Glutathione transferases (GSTs) constitute a widespread superfamily of enzymes notably involved in detoxification processes and/or in specialized metabolism. In the cyanobacterium Synechocsytis sp. PCC 6803, SynGSTC1, a chi-class GST (GSTC), is thought to participate in the detoxification process of methylglyoxal, a toxic by-product of cellular metabolism. GSTCs were shorter of about 30 residues compared to most cytosolic GSTs and had a well-conserved SRAS motif in the active site (10SRAS13 in SynGSTC1). The crystal structure of SynGSTC1 in complex with glutathione adopted the canonical GST fold with a very open active site because the α4 and α5 helices were exceptionally short.

We also solved the structures of two variants (S10T and R11A variants in complex with GSH) which did not show significant differences from the wild-type. The R11A substitution also did not fully abolish the activity of the enzyme even though it decreased significantly (divided by a factor close to 250 as compared to WT). R11 formed a salt bridge with the N-terminal carboxylate group of GSH in the crystal structure (see above in Section 3.3). The electrostatic influence of R11 on the catalytic process was, however, clear since the catalytic rate was 75 times lower in R11A compared to WT. This was accompanied by a significant one-unit increase in optimal pH suggesting a higher GSH-thiol pKa in the R11A variant than in the WT enzyme. The SynGSTC1 residues with the largest contributions were R11, K51, R116, which formed salt bridges with the GSH negative charges. The arginine residue was invariant, the first position was replaced in a few cases by a threonine residue and the last two positions were a bit more variable.

>[2x]MIKLYGAPQSAASIIQWYLEELSLPYEFVNVNLKEGEHRQAPYLAINPFGKVPAIADGNFHLWESGAILLYLAEKASTIPADAQARALVNQWILFANSTLANGLFIEAVREKEMPRLLQSLEKILGRSPFILGEKFSVVDVAVGSILAYVPIMLKLNFDDYPAVAAYVQGLVQRPAFQASIGARLEHHHHHH> MTKKV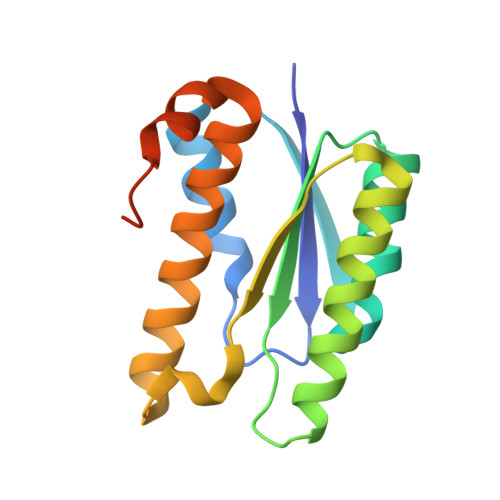GIVDTTFARVDMASAAILTLKMESPNIKIIRKTVPGIKDLPVACKKLLEEEGCDIVMALGMPGKAEKDKVCAHEASLGLMLAQLMTNKHIIEVFVHEDEAKDDAELKILAARRAIEHALNVYYLLFKPEYLTRMAGKGLRQGFEDAGPARE>GSHMGHWSQGLKISMQDPKMQVYKDEQVVVIKDKYPKARYHWLVLPWTSISSLKAVAREHLELLKHMHTVGEKVIVDFAGSSKLRFRLGYHAIPSMSHVHLHVISQDFDSPCLKNKKHWNSFNTEYFLESQAVIEMVQEAGRVTVRDGMPELLKLPLRCHECQQLLPSIPQLKEHLRKHWTQ[2x]

The APTX RNA‐DNA deadenylase protects genome integrity and corrects abortive DNA ligation arising during ribonucleotide excision repair and base excision DNA repair, and APTX human mutations cause the neurodegenerative disorder ataxia with oculomotor ataxia 1 (AOA1). The aprataxin (APTX) RNA/DNA polynucleotide deadenylase directly reverses 5′‐AMP damage (Ahel et al, 2006; Harris et al, 2009; Reynolds et al, 2009; Tumbale et al, 2011, 2014) and associates with DNA repair scaffolds XRCC1 (Cherry et al, 2015) and XRCC4. Environmental and metabolic sources of DNA damage prompt “abortive ligation”, the failure of ligase to complete step 3, and generation of 5′‐adenylated (5′‐AMP) DNA strand breaks (Ahel et al, 2006; Andres et al, 2015; Schellenberg et al, 2015). AOA1 mutations map to the APTX catalytic domain (Barbot et al, 2001; Moreira et al, 2001; Shimazaki et al, 2002; Le Ber et al, 2003; Tranchant et al, 2003; Criscuolo et al, 2004, 2005; Ito et al, 2005; Mosesso et al, 2005; Baba et al, 2007; Yokoseki et al, 2011) and cause variable age of disease onset.

We obtained crystals diffracting to 2.4 Å resolution that contain two APTX catalytic domain (APTXcat, residues 165–342) protomers engaging a doubly nicked target structure. Successful crystallization strategies ultimately utilized a concatemerized nick substrate with a 6 bp upstream and 8 bp downstream duplexes. In addition, a 5′‐ribonucleotide is positioned at the nick junction. In this configuration, the structural snapshots captured in our crystal structures are representative of APTX bound to a nicked RNA‐5′‐3′‐DNA junction reaction product complex formed by APTX during repair of abortive ligation products created during ribonucleotide excision repair (RER) (Tumbale et al, 2014; Schellenberg et al, 2015). The structure reveals how APTX induces large‐scale DNA duplex substrate distortions in order to access the 5′‐terminal adenylated lesion in the context of a nicked duplex. The major molecular interface at the DNA nick is mediated by the amino‐terminal HIT domain α‐helix (α1) that infiltrates the DNA base stack. The planar rings of His166 and Trp167 together redirect the DNA duplex, imparting a ~90° bend to the substrate RNA‐DNA. The protein displaces the upstream half of the nick and unwinds both the 3′ and 5′ sides of the nick. This has two effects: First, extraction of the 5′‐terminus facilitates positioning of the adenylated lesion into the active site; and second, disruption of the 3′‐terminal side of the nick exposes the 3′ end. In each of the complexes captured in our crystals, abrupt DNA bending is governed by the APTX amino‐terminal helix, as previously hypothesized (Tumbale et al, 2011). This structure illuminates how APTX senses DNA damage through two discontinuous nucleic acid binding sub‐sites, dictated by both the HIT and Znf domains which together collaborate to sense the nick.>[4x]MGLSLPKEKGLILCLWSKFCRWFQRRESWAQSRDEQNLLQQKRIWESPLLLAAKDNDVQALNKLLKYEDCKVHQRGAMGETALHIAALYDNLEAAMVLMEAAPELVFEPMTSELYEGQTALHIAVVNQNMNLVRALLARRASVSARATGTAFRRSPCNLIYFGEHPLSFAACVNSEEIVRLLIEHGADIRAQDSLGNTVLHILILQPNKTFACQMYNLLLSYDRHGDHLQPLDLVPNHQGL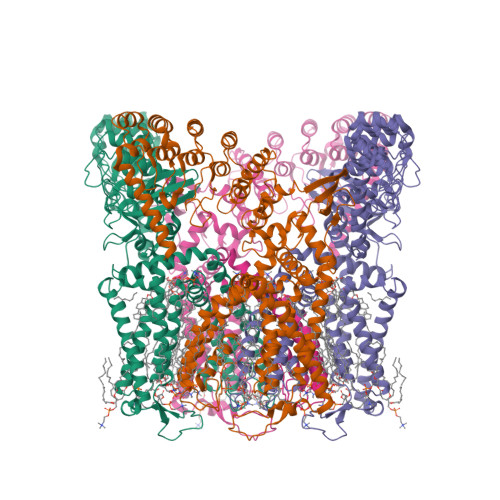TPFKLAGVEGNTVMFQHLMQKRKHTQWTYGPLTSTLYDLTEIDSSGDEQSLLELIITTKKREARQILDQTPVKELVSLKWKRYGRPYFCMLGAIYLLYIICFTMCCIYRPLKPRTNNRTSPRDNTLLQQKLLQEAYMTPKDDIRLVGELVTVIGAIIILLVEVPDIFRMGVTRFFGQTILGGPFHVLIITYAFMVLVTMVMRLISASGEVVPMSFALVLGWCNVMYFARGFQMLGPFTIMIQKMIFGDLMRFCWLMAVVILGFASAFYIIFQTEDPEELGHFYDYPMALFSTFELFLTIIDGPANYNVDLPFMYSITYAAFAIIATLLMLNLLIAMMGDTHWRVAHERDELWRAQIVATTVMLERKLPRCLWPRSGICGREYGLGDRWFLRVEDRQDLNRQRIQRYAQAFHTRGSEDLDKDSVEKLVPRGSAAAWSHPQFEK>MIPKTKAEGVPDFVLLNQITENAFIENLTMRHKSDNIYTYIGDVVISTNPFKNLNIYKESDIKAYNGRYKYEMPPHMYALANDAYRSMRQSQENQCVIISGESGAGKTEASKKIMQFLTFVSSNQSPNGERISKMLLDSNPLLEAFGNAKTLRNDNSSRFGKYMEMQFNAVGSPIGGKITNYLLEKSRVVGRTQGERSFHIFYQMLKGLSQSKLDELGLTPNAPAYEYLKKSGCFDVSTIDDSGEFKIIVKAMETLGLKESDQNSIWRILAAILHIGNITFAEAAEQRTGTTTVKVSDTKSLAAAASCLKTDQQSLSIALCYRSISTGVGKRCSVISVPMDCNQAAYSRDALAKALYERLFNWLVSKINTIINCTTEKGPVIGILDIYGFEVFQNNSFEQLNINFCNEKLQQLFIELTLKSEQEEYVREGIEWKNIEYFNNKPICELIEKKPIGLISLLDEACLIAKSTDQTFLDSICKQFEKNPHLQSYVVSKDRSIGDTCFRLKHYAGDVTYDVRGFLDKNKDTLFGDLISSMQSSSDPLVQGLFPPTRPEDSKKRPETAGSQFRNAMNALITTLLACSPHYVRCIKSNDNKQAGVIDEDRVRHQVRYLGLLENVRVRRAGFAGRIEYTR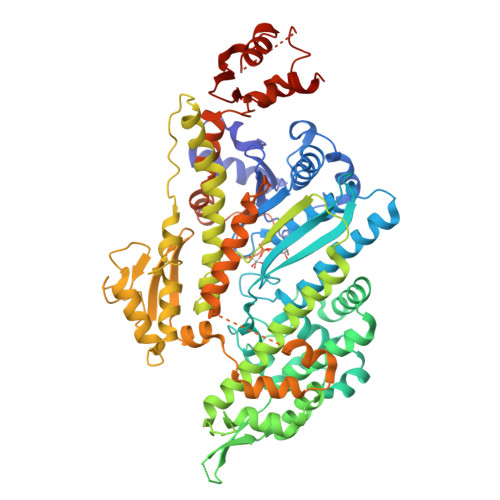FYNRYKMLCKKTWPSFNGTAKQATELILQQHNIDKEEIRMGKTKVFIRNPTTLFYFEEKRELEMP[4x]> MNIPQRQFSNEEVNRCYLRWQHLRNEHGMNAPSVPEFIYLTKVLQFAAKQRQELQMQRQQQGISGSQQNIVPNSSDQAELPNNASSHISASASPHLAPNMQLNGNETFSTSAHQSPIMQTQMPLNSNGGNNMLPQRQSSVGSLNATNFSPTPANNGENAAEKPDNSNHNNLNLNNSELQPQNRSLQEHNIQDSNVMPGSQINSPMPQQAQMQQAQFQAQQAQQAQQAQQAQQAQARLQQGRRLPMTMFTAEQSELLKAQITSLKCLVNRKPIPFEFQAVIQKSINHPPDFKRMLLSLSEFARRRQPTDQNNQSNLNGGNNTQQPGTNSHYNNTNTDNVSGLTRNAPLDSKDENFASVSPAGPSSVHNAKNGTLDKNSQTVSGTPITQTESKKEENETISNVAKTAPNSNKTHTEQNNPPKPQKPVPLNVLQDQYKEGIKVVDIDDPDMMVDSFTMPNISHSNIDYQTLLANSDHAKFTIEPGVLPVGIDTHTATDIYQTLIALNLDTTVNDCLDKLLNDECTESTRENALYDYYALQLLPLQKAVRGHVLQFEWHQNSLLTNTHPNFLSKIRNINVQDALLTNQLYKNHELLKLERKKTEAVARLKSMNKSAINQYNRRQDKKNKRLKFGHRLIATHTNLERDEQKRAEKKAKERLQALKANDEEAYIKLLDQTKDTRITHLLRQTNAFLDSLTRAVKDQQKYTKEMIDSHIKEASEEVDDLSMVPKMKDEEYDDDDDNSNVDYYNVAHRIKEDIKKQPSILVGGTLKDYQIKGLQWMVSLFNNHLNGILADEMGLGKTIQTISLLTYLYEMKNIRGPYLVIVPLSTLSNWSSEFAKWAPTLRTISFKGSPNERKAKQAKIRAGEFDVVLTTFEYIIKERALLSKVKWVHMIIDEGHRMKNAQSKLSLTLNTHYHADYRLILTGTPLQNNLPELWALLNFVLPKIFNSVKSFDEWFNTPFANTGGQDKIELSEEETLLVIRRLHKVLRPFLLRRLKKDVEKELPDKVEKVVKCKMSALQQIMYQQMLKYRRLFIGDQNNKKMVGLRGFNNQIMQLKKICNHPFVFEEVEDQINPTRETNDDIWRVAGKFELLDRILPKLKATGHRVLIFFQMTQIMDIMEDFLRYINIKYLRLDGHTKSDERSELLRLFNAPDSEYLCFILSTRAGGLGLNLQTADTVIIFDTDWNPHQDLQAQDRAHRIGQKNEVRILRLITTNSVEEVILERAYKKLDIDGKVIQAGKFDNKSTSEEQEALLRSLLDAEEERRKKRESGVEEEEELKDSEINEILARNDEEMAVLTRMDEDRSKKEEELGVKSRLLEKSELPDIYSRDIGAELKREESESAAVYNGRGARERKTATYNDNMSEEQWLRQFEVSDDEKNDKQARKQRTKKEDKSEAIDGNGEIKGENIDADNDGPRINNISAEDRADTDLAMNDDDFLSKKRKAGRPRGRPKKVKLEGSENSEPPALESSPVTGDNSPSEDFMDIPKPRTAGKTSVKSARTSTRGRGRGRGRGRGRGRGRGRPPKARNGLDYVRTPAAATSPIDIREKVAKQALDLYHFALNYENEAGRKLSDIFLSKPSKALYPDYYMIIKYPVAFDNINTHIETLAYNSLKETLQDFHLIFSNARIYNTEGSVVYEDSLELEKVVTKKYCEIMGDNSQLDFTEFDEQYGTRPLVLPPVVTSSVAESFTDEADSSMTEASV;> MDFFNLNNNNNNNNTTTTTTTTNNNNTNNNNTNNNNNPANNTNNNNSTGHSSNTNNNTNNNNTNTGASGVDDFQNFFDPKPFDQNLDSNNNNSNSNNNDNNNSNTVASSTNFTSPTAVVNNAAPANVTGGKAANFIQNQSPQFNSPYDSNNSNTNLNSLSPQAILAKNSIIDSSNLPLQAQQQLYGGNNNNNSTGIANDNVITPHFITNVQSISQNSSSSTPNTNSNSTPNANQQFLPFNNSASNNGNLTSNQLISNYAASNSMDRSSSASNEFVPNTSDNNNNSNNHNMRNNSNNKTSNNNNVTAVPAATPANTNNSTSNANTVFSERAAMFAALQQKQQQRFQALQQQQQQQQNQQQQNQQPQQQQQQQQNPKFLQSQRQQQQRSILQSLNPALQEKISTELNNKQYELFMKSLIENCKKRNMPLQSIPEIGNRKINLFYLYMLVQKFGGADQVTRTQQWSMVAQRLQISDYQQLESIYFRILLPYERHMISQEGIKETQAKRIFLQQFLQELLKKVQQQQQAAALANANNNINSASSAPTPAAPGASVPATAAPGTEAGIVPVSANTPKSLNSNININVNNNNIGQQQVKKPRKQRVKKKTKKELELERKEREDFQKRQQKLLEDQQRQQKLLLETKLRQQYEIELKKLPKVYKRSIVRNYKPLINRLKHYNGYDINYISKIGEKIDSNKPIFLFAPELGAINLHALSMSLQSKNLGEINTALNTLLVTSADSNLKISLVKYPELLDSLAILGMNLLSNLSQNVVPYHRNTSDYYYEDAGSNQYYVTQHDKMVDKIFEKVNNNATLTPNDSNDEKVTILVDSLTGNQLPTPTPTEMEPDLDTECFISMQSTSPAVKQWDLLPEPIRFLPNQFPLKIHRTPYLTSLKKIKDEIDDPFTKINTRGAEDPKVLINDQLSTISMILRNISFSDNNSRIMSRNFYLKRFISDLLWLVLIHPENFTCNRKILNFKKDLVIVLSNISHLLEIASSIDCLLILILVISFGQPKLNPMASSSSFGSESLTFNEFQLQWGKYQTFGVDILAKLFSLEKPNLNYFKSILLNKNTGNNLYDRNSNNNHKDKKLLRRLLNLYNDNNKNNNNRHNLLNDVVSFLFSAIPLQQVLSQSADPSLLIDQFSPVISQSLTSILVIVQKILPLSNEVFEISENNSDSNSNNNGNKDSSFNFNKNLPFVWLSSEENIGSGLLKLSEIILNINNSTSKNTLLQQQNYSKVLLPSINISCVQLIKCLVEKSICFENCLNNDPEILKKIASIPNLFPTDLEIFQLFTNPSVDIQIINQYQLLYNLKNDILTNLE;> MNNQPQGTNSVPNSIGNIFSNIGTPSFNMAQIPQQLYQSLTPQQLQMIQQRHQQLLRSRLQQQQQQQQQTSPPPQTHQSPPPPPQQSQPIANQSATSTPPPPPAPHNLHPQIGQVPLAPAPINLPPQIAQLPLATQQQVLNKLRQQAIAKNNPQVVNAITVAQQQVQRQIEQQKGQQTAQTQLEQQRQLLVQQQQQQQLRNQIQRQQQQQFRHHVQIQQQQQKQQQQQQQHQQQQQQQQQQQQQQQQQQQQQQQQQQQQQQQQQQQQQGQIPQSQQVPQVRSMSGQPPTNVQPTIGQLPQLPKLNLPKYQTIQYDPPETKLPYPTYWSDKKADTDTLLYEQIIQRDKINKYSLIRETNGYDPFSIYGFSNKEYISRLWHTLKYYQDLKNTRMKSITSTSQKIPSASIWGNGYSGYGNGITNTTTRVIPQVEVGNRKHYLEDKLKVYKQAMNETSEQLVPIRLEFDQDRDRFFLRDTLLWNKNDKLIKIEDFVDDMLRDYRFEDATREQHIDTICQSIQEQIQEFQGNPYIELNQDRLGGDDLRIRIKLDIVVGQNQLIDQFEWDISNSDNCPEEFAESMCQELELPGEFVTAIAHSIREQVHMYHKSLALLGYNFDGSAIEDDDIRSRMLPTITLDDVYRPAAESKIFTPNLLQISAAELERLDKDKDRDTRRKRRQGRSNRRGMLALSGTSASNTSMNGVHNTVAAGNASSLPPGEILLPDIADIPRTFRTPVPSTLMPGGVDVGPSVESYELRNTTTYKSRPDRPKPVSPPCYIIDHIPGHSLLLSIKLPGKVNTKEEFAAAPNDTSSGTNAMLPSPESLKTKLNSNIRAGVTIPSIPNPIANHTVTNSPNPTLQPVIPGGAASKSVPTPSLPIAPPVAPHDSEATLLTNSNNGSSNNNTQNT;>MENTLGEGSTVNASVDVDQHGNDNNSDSNANAAVAGVANTDTAGEESQQQDESLKDEATVPNTRDAESEAITVTAKQQPTMQANKLDSQETPSTEESRAQNVFGQDNEDSDNLFGETESSVSNNEANTPSIPTNPVDNENNKPAIKEDSTIQDSNGDVKNMEDVKIQKEEEPENNTVIEGVKEESQPDENTKEMDEVEEDDEDDDQPMISPDNSIFGDTKSESKQLGNTSSVANTPSEIPDAHKAEQEDIIEKTESVDKKVDSGEERNEQEREIMNDHSKSANPKKTTITRVEPETFEIPQAHEIVIPSYSKWFNLEKIHSIEVQSLPEFFTNRIPSKTPEVYMRYRNFMVNSYRLNPNEYFSVTTARRNVSGDAAALFRLHKFLTKWGLINYQVDSKLLPKNIEPPLTSQYSTRHDAPRGLFPFESYKPSVQLPDMAKLKKMMNTSDSESTLYKYLKESKRKYDEITHPPSTTDDENGDKNDNGGKMNNEVSTSTSMTGDANLLEEGETSRPLKKVKILEQIDENWSKEDLQKLLKGIQEFGADWYKVAKNVGNKSPEQCILRFLQLPIEDKFLYGDGNGKGDNDNGLGPLKYAPHLPFSKSENPVLSTIAFLVGLVNPKTVQSMTQRAIQSAESIKSQKEEISDQKPIEHIKEGSEIAISSLGYRSHIFATNEERQMNFLTNELIRLQMEKLDAKLNHLKKLEKFMELERKTLERQQENLLIQRLNFNQNSSKIVNVLSKCLNLISDSNINNSSVAEKEEIRSQIDHFKSMLSKPETLSIGKNPFNKPNIETGENHNGQSISNENDVKPISIEAPQFYRYWSA[4x];> MSKVMKPSNGKGSRKSSKAATPDTKNFFHAKKKDPVNQDKANNASQITPTVPHSHPSDM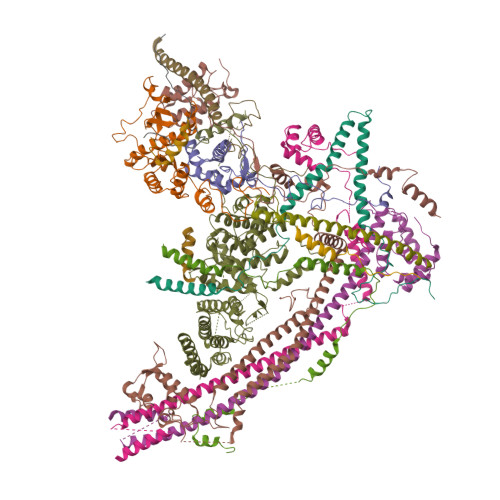VIPDHLAELIPELYSFQQLVDSEKRLDHFIHLRNLHMKRMVAQWERSKLSQEFLYPHLNFPNVKFLRIFISNVSENQPWQMDTNNEADLMALENATWTMRIEGRLLDNVQANDPAREKFSSFIESIVVDFKNKENDNVPSTKFNAAPEENATEGPSDKKLNLNLPLQFSLPNGDNSTTTNTDQNNATMGEETAKKDMSSTTPKLESVKWQYDPNNPVDFDGLDIKRVGSENVECTISILRKSSPEEPFMSYSPQLTAIIGLKSGTSHDAIFSIYKYIHLNELLTNDESAFENLMGNRNNHNSNTSTSKMLDAASSQVSIVKLDTQLITLLPSSLKESSPDTMKLTDLLSLINSTHLLPLQPIEIDYTVRVDKASTYGELVLDIEVPDVNALKFNNTQRESQIGAAELNENARELEQIKPKIALQDKEITSVLSNLHESNKRYRFFKKISEDPVKALNECIASTSNALKVLSGDEGYNEDMVRRANFYKENEAMLRENIEVILSNGRM;> MGVIKKKRSHHGKASRQQYYSGVQVGGVGSMGAINNNIPSLTSFAEENNYQYGYSGSSAGMNGRSLTYAQQQLNKQRQDFERVRLRPEQLSNIIHDESDTISFRSNLLKNFISSNDAFNMLSLTTVPCDRIEKSRLFSEKTIRYLMQKQHXXXXXXXXXXXXXXXXXXXXXXXXXXXXX1-methyl-9~{H}-pyrido[3,4-b]indol-7-ol 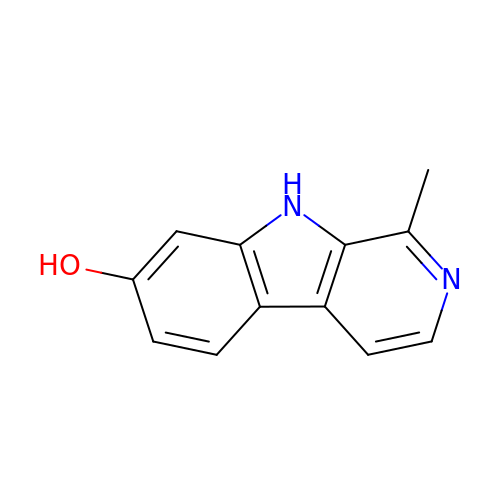| C12 H10 N2 O | SATMZMMKDDTOSQ-UHFFFAOYSA-N In PT-based Dnd defense systems, DndABCDE serves as the modification component to catalyze double-stranded DNA PT modification at the 5′-GPSAAC-3′/5′-GPSTTC-3′ sites (PS, phosphate-sulfur linkage), while DndFGH utilizes sequence-specific PT modification as the recognition tag to discriminate against and eliminate invasive foreign DNA lacking PT modification. Although it has been confirmed that iscS-dndBCDE and dndFGH form an antiphage defense system, in this study, we found that a dndI gene, situated within the dndFGHI operon, also constitutes a PT-based antiphage defense system along with the iscS-dndBCDE module. Sequence analysis reveals that DndI comprises an N-terminal DUF262 and a C-terminal DUF1524 His-Asn-His (HNH) nuclease domain, similar to the domain organization in SspE. Upon sensing PT modifications at 5′-GPSAAC-3′/5′-GPSTTC-3′, the ATPase activity of DndI is stimulated, which subsequently triggers a conformational transition, facilitating the dissociation of DndI from self-DNA, thereby allowing DndI to avoid cleaving self-DNA while restricting PT-deficient phage DNA.

Moreover, we resolved the crystal structure of DndI from Salmonella at a resolution of 3.10 Å. In each asymmetric unit, DndI forms a homodimer, where each protomer of DndI consists of a smaller N-terminal domain (residues 1–238, hereinafter DndINTD) and a larger C-terminal domain (residues 239–596, hereinafter DndICTD). The conserved D83GQQR87 motif, a key motif for NTP hydrolysis, is located at the junction of the α3 helix and the β3 sheet of DndINTD. Unlike the typical HNH motif observed in Colicin E9 (39), ScoMcrA, Cas9 (41), BrxU and Ref, which is composed of an α-helix and two antiparallel β-strands, the HNH motif located in DndICTD consists of two β-strands and a loop, showing similarities to the HNH motif found in SspE of Streptomcyes yokosukanensis DSM 40224 (27). The CTDs of DndI and SspE exhibit a lower extent of structural similarity (with an RMSD of 4.9 Å for 325 Cα atoms) in comparison to the NTDs (with an RMSD of 3.0 Å for 219 Cα atoms). Significantly, the Y25 residue, which is equivalent to Y30 that mediates the PT responsiveness in SspE from S. yokosukanensis DSM 40224, was situated in a hydrophobic cavity within the N-terminal ATPase domain of DndI. The immediate finding was that the DndIY25A variant with a single-point alanine substitution at Y25 still exhibited intrinsic ATP hydrolysis activity comparable to wild-type DndI but was no longer enhanced by PT modification, suggesting that the Y25-containing hydrophobic patch mediates the responsiveness of DndI to PT markers. To further understand how PT modification modulates other enzymatic activities of DndI, electrophoretic mobility shift assay (EMSA) was conducted, which showed that the binding affinity of DndICTD with DNA (Kd = 0.66 μM) was 14-fold greater than that of full-length DndI (Kd = 9.31 μM), indicating the inhibitory impact of the NTD on the CTD.

>[2x]MNVKPEYMSFGELFKNSNIFYTPTYQRDYSWEDEQIEQFCNDIQDALVKKKSKKSCEHFFGGVVCAQEKTFGGHRRIENLLVDGQQRLSTIVLFFSVIRNVINSLNCEEDKDSEYRGMILKDIYKYFYLDERENREIKKHVRITIGNADNEFYQSLIDDNPLKGTRNSHELMLRARKKFNSFIKDDLFKNRKISECLEIIDDIVKLFEESFLVIHIVTNSIDDAYKLFTVLNDRGINLTEGELLKAHTIGICSDNLSHQRTISDNWDAILKHPSKKVTDYLRWILIMLTGNNITASSVLEEYKKTVFNELISKSEIAQTVAYIRDCVERLEYISSGEWPFENNNDNKWHKSKLDLLINKLKHLHAMPLLLAASFSSENNFKHIVNETSKFFIRCKMISDLHASIFSKLYAVLALRIHKERDRFDISKLHGAFNEILLDKDPEDVRFSTNVRSLIYQKKGDNKPIKCLLMTIQENWEWLKQPCQGNSLNRLKREDQTIIFDFNSMTLEHIYPYSALHEDKDMDMEKLKNNIGNIVLLDPTRNNKNDNKPFIDKKNSFENTGIGIHSWIYEQKEWTEESVKKLTETYVDAAVKVFSFS One DNA transposon, Hsmar1, was active in primates from about 50 to 37 million years ago and gave rise to SETMAR (or Metnase), a fusion protein found only in simian (anthropoid) primates with an N-terminal SET domain and C-terminal Hsmar1-derived (MAR) transposase. SETMAR comprises three structural domains, a SET domain, a transposase-derived DBD, and a catalytic domain. The first is retention of ancestral sequence-specific TIR-DNA-binding activity, mediated by the DNA-binding domain (DBD) of the transposase, although the ability to perform TIR-specific DNA cleavage events has been lost. The second SETMAR function is lysine methyltransferase (KMT) activity, which is contained within the SET domain.

To provide a structural basis for recognition of TIR-DNA by SETMAR, we used a selenomethionine (SeMet) phasing strategy to determine the crystal structure of the SETMAR DBD comprising residues 329 to 440 complexed to a 25-mer DNA derived from the Hsmar1 TIR at 2.37 Å resolution. Thus as previously reported, a phasing strategy was devised in which strategic Met substitutions (I359M) (L423M) within two predicated alpha helical elements were introduced; these Met substitutions were critical for phasing. The C381R substitution was introduced to prevent disulfide bond formation. The structure of the complex is dimeric with two DBDs, each bound to a TIR-DNA duplex oriented in parallel to one another; the DBD comprises two helix–turn–helix (HTH) motifs connected by a 17 amino acid residue linker (residues 384–400) containing two AT hook elements bound to the 25-mer TIR DNA duplex. A relatively large surface area (1610 Å2) involving interactions of F344, F363, and I341 in each HTH1 motif is buried in the dimer interface. Sequence-specific recognition of the 19 bp TIR element (5′-GGTGCAAAAGTAATTGCGG) is mediated by 32 hydrogen-bonding interactions, nine in the major groove (two in HTH1 and seven in HTH2), five in the minor groove from the AT-hook elements within the linker, and 18 with the phosphodiester backbone. Within HTH1, the larger of the two HTH motifs, a single residue, R371 in recognition helix α3, forms two nucleobase-specific hydrogen bonds with G5 (B chain). From HTH2, S428 and R432 of recognition helix α6 hydrogen bond to C18 and G17 (B chain) and G8 and C9 (C chain); R417 and H427 hydrogen bond to G5 and G6 (C chain), respectively. Within the central AT-rich regions of the TIR, R392 and R395 act as two AT hooks forming specific hydrogen bonds to nucleobases in the minor groove. Individual substitution of Ala for R371, S428, or R432 located in the recognition helices in FL SETMAR resulted in significant decreases in affinity with relative KD values for binding of WT, R371A, S428A, and R432A to TIR DNA of 42 ± 5, 521 ± 65, 485 ± 58, and 302 ± 47 nM, respectively.

> SMKMMLDKKQIRAIFLFEFKMGRKAAETTRNMNNAFGPGTANERTVQWWFKKFRKGDESLEDEERSGRPSEVDNDQLRAIIEADPLTTTREVAEEMNVNHSTVVRHLKQIGKV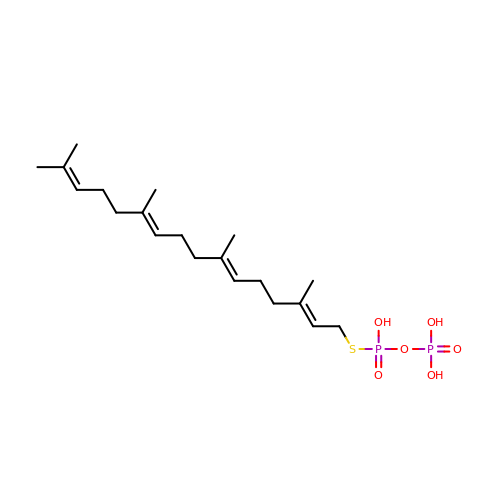phosphonooxy-[(10E)-3,7,11,15-tetramethylhexadeca-2,6,10,14-tetraenyl]sulfanyl-phosphinic acid | C20 H36 O6 P2 S | BUSOKXFDTDWPOS-OGGZDJOISA-N>MKNNGGARVVVIGAGFVGASYVFALMNQGIADEIVLIDANESKAIGDAMDFNHGKVFAPKPVDIWHGDYDDCRDADLVVICAGANQKPGETRLDLVDKNIAIFRSIVESVMASGFQGLFLVATNPVDILTYATWKFSGLPHERVIGSGTILDTARFRFLLGEYFSVAPQNVHAYI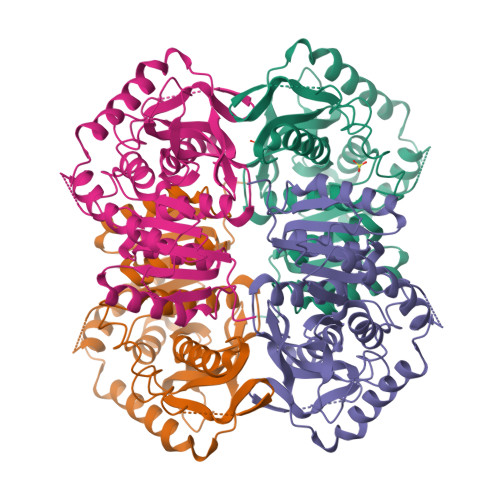IGEHGDTELPVWSQAYIGVMPIRKLVESKGEEAQKDLERIFVNVRDAAYQIIEKKGATYYGIAMGLARVTRAILHNENAILTVSAYLDGLYGERDVYIGVPAVINRNGIREVIEIELNDDEKNRFHHSAATLKSVLARAFTR[4x]> DWISFSHMSSDTDHFPIKSWFRCEQKAASRSYRTLGDMSHPQGIYEVRAAITRLISLTRGVKCRPEQMIIGAGTQVLMQLLTELLPKEAVYAMEEPGYRRMYQLL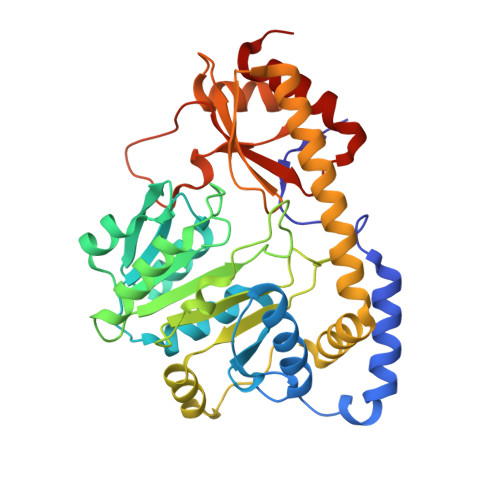KNAGKQVKTIMLDEKGMSIAEITRQQPDVLVTTPSHQFPSGTIMPVSRRIQLLNWAAEEPRRYIIEDDYDSEFTYDVDSIPALQSLDRFQNVIYMGTFSKSLLPGLRISYMVLPPELLRAYKQRGYDLQTCSSLTQLTLQEFIESGEYQKHIKKMKQHYKEKRERLITALEAEFSGEVTVKGANAGLHFVTEFDTRRTEQDILSHAAGLQLEIFGMSRFNLKENKRQTGRPALIIGFARLKEEDIQEGVQRLFKAVYGHR> GFGNQGGFGNSRGGGAGLGNNQGSNMGGGMNFGAFSINPAMMAAAQAALQSSWGMMGMLASQ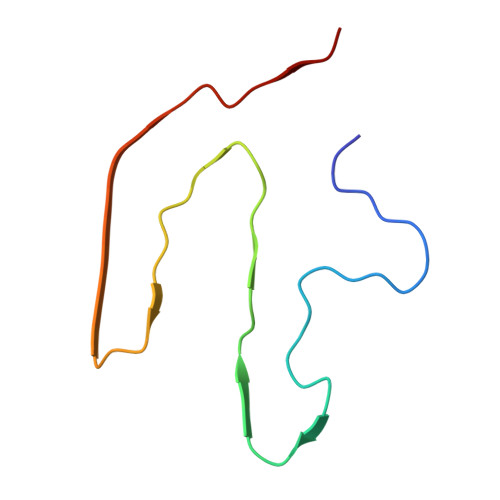QN> GAMVSPSLIAKFEKTSKSNIEGTIKFTPANNGTVSVSVDLKGLPSDIGPFPYHVHEKPVPASKNCSATENHFNPYNGTVRAATPAAHEVGDLAGKHGNIMGESYKTEYDDSYISLNEKSRSYIGGLSIVIH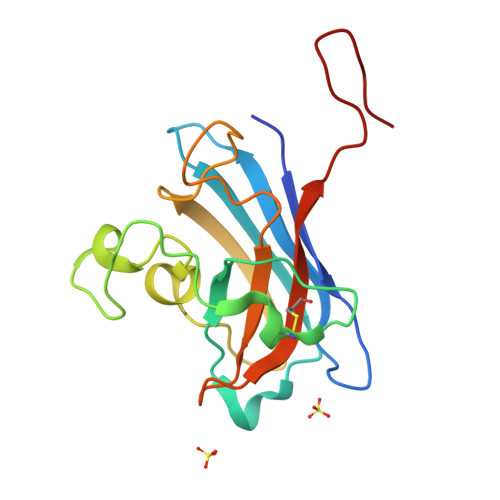ANNGTRLNCANITLLDEGHGNANTTMSN Type IIB receptor protein tyrosine phosphatases are cell surface transmembrane proteins that engage in cell adhesion via their extracellular domains (ECDs) and cell signaling via their cytoplasmic phosphatase domains. The four human R2B RPTPs (PTPRK, PTPRM, PTPRT, and PTPRU) are type 1 transmembrane proteins and share a common extracellular domain (ECD) architecture of one MAM (meprin/A5/μ), one immunoglobulin (Ig)-like, and four fibronectin (FN) type-III domains, with the most membrane proximal FN domain undergoing furin cleavage in the secretory pathway. Previous studies have shown that PTPRK, PTPRM, and PTPRT form homodimers, but not heterodimers, in cell aggregation assays. The homophilic (trans) interactions of R2B RPTPs determine their subcellular localization and have been proposed to function as spacer clamps between cell membranes.

Here, we have solved the X-ray crystal structure of the membrane-distal N-terminal domains of PTPRK that form a head-to-tail dimer consistent with intermembrane adhesion. The structure comprises a MAM domain (residues 31–192) that forms an extensive intramolecular interface with the Ig domain (residues 193–290), followed by the FN1 domain (residues 291–388) that makes few interdomain contacts with the Ig domain (discussed later). Three glycosylation sites were observed in the electron density maps at asparagine residues N101 and N140 in the MAM domain and N211 in the Ig domain. Two chains of PTPRK-MIFN1 were present in the asymmetric unit of the crystal structure forming a head-to-tail dimer and burying a surface area of ∼1750 Å2. The dimer interface is formed between the MAM–Ig domain from one molecule and the FN1 domain of the opposing molecule, similar to that observed previously for PTPRM. Notably, the orientation of the W160MAM carbonyl oxygen is caused by a cis-peptide bond with the adjacent P161MAM, a conformation that is stabilized by the side chain of W160MAM stacking with the N-acetylglucosamine of the N101MAM glycan. Both W351FN1 and H352FN1 occupy a deep groove located at the MAM–Ig boundary of the opposing molecule, burying ∼90% of their solvent-accessible surface area. All but one of these key residues are completely conserved across the R2B receptor ECDs, the difference being that PTPRK W351FN1 is a glycine in PTPRM. Mutation of W351 in PTPRK to glycine significantly disrupts dimerization but does not completely abolish it. Detailed comparison of the PTPRK-MIFN1 structure with the equivalent region of PTPRM reveals a significant hinge movement (approximately 15°) of the FN1 domain relative to the MAM–Ig domains. The differing MIFN1 interdomain orientations result in low shape complementarity for the modeled PTPRK–PTPRM dimer interface (Sc = 0.206) when compared with the homodimer structures (Sc = 0.581 for PTPRK and 0.575 for PTPRM).

>[2x]ETGQGQFSAGGCTFDDGPGACDYHQDLYDDFEWVHVSAQEPHYLPPEMPQGSYMIVDSSDHDPGEKARLQLPTMKENDTHCIDFSYLLYSQKGLNPGTLNILVRVNKGPLANPIWNVTGFTGRDWLRAELAVSTFWPNEYQVIFEAEVSGGRSGYIAIDDIQVLSYPCDKSPHFLRLGDVEVNAGQNATFQCIATGRDAVHNKLWLQRRNGEDIPVAQTKNINHRRFAASFRLQEVTKTDQDLYRCVTQSERGSGVSNFAQLIVREPPRPIAPPQLLGVGPTYLLIQLNANSIIGDGPIILKEVEYRMTSGSWTETHAVNAPTYKLWHLDPDTEYEIRVLLTRPGEGGTGLPGPPLITRTKGTKHHHHHH> GSHMMADLLPRVDIAPQITEALLKEMSDKDWKTRNEGLTKLQAIISEARLIKPSIGDLAPALAHRLVDSNAKIAQTTLAICEQLATAMGAGCRNHVRNLFPGFLHALGDNKSFVRAAALNCINSFGEKGGYKEFFESEMIADALKGGSPALKTELWAWLADKL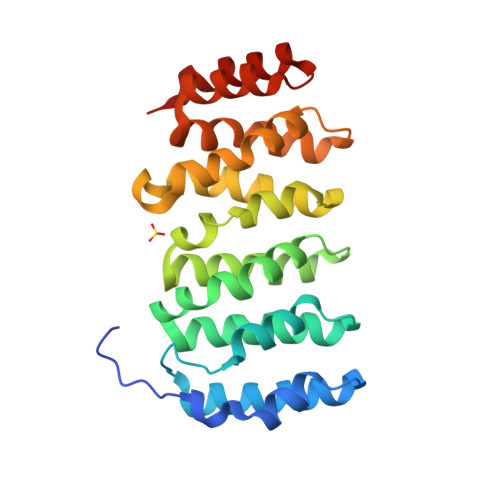PGLPPKSVSKEDIHSMVPHLYAHICDRNADVRKNANEAVLGIMIHLGFDAMNRALDKQKPASKKDILAALEKARPNLP> YSDPKEYIESKYYDALFSIHTPLAYFVKSNLVRLKNTCRTKYGSDSYKIAYQAMLQ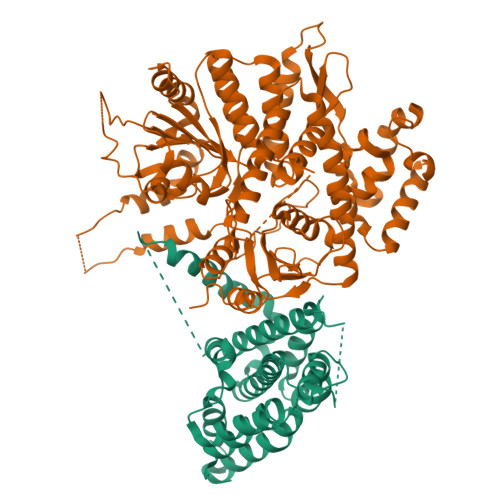KFLLSIVQFKDRHDNRLLLEPFSSPIADEKRKNCLTKFVIQDENKNSSTIADLCVVLKSREIKLQILLLLEIIGLNDLDWNFRDFEKKYKLKLKKRSLNLTKKGLVRRRSKKKTSEKDKGIERITTSLDYCEQLDLYLDRACILDILLSSETPNPDAIEASNGTIQEHKKNILDKSKEASLVGFINYVLIPYFNKKVPHAVEFIIQKLKGP;> MYYGISQFSEAYNKILRNSSSHSSCQLVIFVSCLNIDALCATKMLSLLFKKQLVQSQIVPIFGYSELRRHYSQLDDNINSLLLVGFGGVIDLEAFLEIDPQEYVIDTDEKSGEQSFRRDIYVLDAHRPWNLDNIFGSQIIQCFDDGTVDDTLGEQKEAYYKLLELDEESGDDELSGDENDNNGGDDEATDADEVTDEDEEDEDETISNKRGNSSIGPNDLSKRKQRKKQIHEYEGVLEEYYSQGTTVVNSISAQIYSLLSAIGETNLSNLWLNILGTTSLDIAYAQVYNRLYPLLQDEVKRLTPSSRNSVKTPDTLTLNIQPDYYLFLLRHSSLYDSFYYSNYVNAKLSLWNENGKKRLHKMFARMGIPLSTAQETWLYMDHSIKRELGIIFDKNLDRYGLQDIIRDGFVRTLGYRGSISASEFVEALTALLEVGNSTDKDSVKINNDNNDDTDGEEEEDNSAQKLTNLRKRWVSNFWLSWDALDDRKVELLNRGIQLAQDLQRAIFNTGVAILEKKLIKHLRIYRLCVLQDGPDLDLYRNPLTLLRLGNWLIECCAESEDKQLLPMVLASIDENTDTYLVAGLTPRYPRGLDTIHTKKPILNNFSMAFQQITAETDAKVRIDNFESSIIEIRREDLSPFLEKLTLSGLL>MAQSLQDQTNLHNKLIGEVMKISDQHSQAFVAKLMEQMQQQQLLMSKEIQTNLQVIEENNQRHKAMLDSMQEKFATIIDSSLQSVEEHAKQMHKKLEQLGAMSLPDAEELQNLQEELANERALAQQEDALLESMMMQMEQIKNLRSKNSISMSVHLNKMEESRLTRNHRIDDIKSGIQDYQKLGIEASQSAQAELTSQMEAGMLCLDQGVANCSMLQVH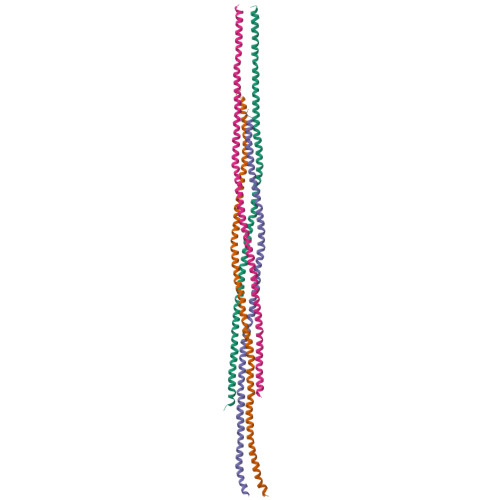MKNLNQKYEKETNENVGSVRVSGHHHHHH[4x]> RANDAPIVLLHGFTGWGREEMFGFKYWGGVRGDIEQWLNDNGYRTYTLAVGPLSSNWDRA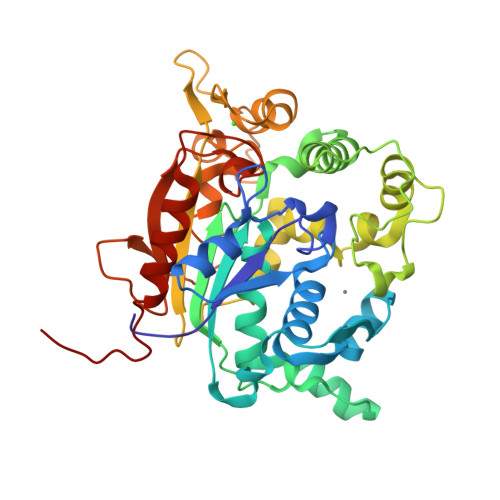CEAYAQLVGGTVDYGAAHAAKYGHARFGRTYPGLLPELKRGGRIHIIAHSQGGQTARMLVSLLENGSQEEREYAKAHNVSLSPLFEGGHHFVLSVTTIATPHDGTTLVNMVDFTDRFFDLQKAVLKAAAVASNVPYTSQVYDFKLDQWGLRRQPGESFDQYFERLKRSPVWTSTDTARYDLSVPGAEKLNQWVKASPNTYYLSFTTERTYRGALTGNYYPELGMNAFSAVVCAPFLGSYRNATLGIDDRWLENDGIVNAFSMNGPKRGSTDRIVPYDGTIKKGVWNDMGTYNVDHLEVIGVDPNPLFDIWAFYLRLAEQLASLQPHHHHHH> EAGAPCGRISFALRYLYGSDQLVVRILQALDLPAKDSNGFSDPYVKIYLLPDRKKKFQTKVHRKTLNPIFNETFQFSVPLAELAQRKLHFSVYDFDRFSRHDLIGQVVLDNLLELAEQPPDRPLWRDILEGGSEKADLGELNFSLCYLPTAGLLTVTIIKASNLKAMD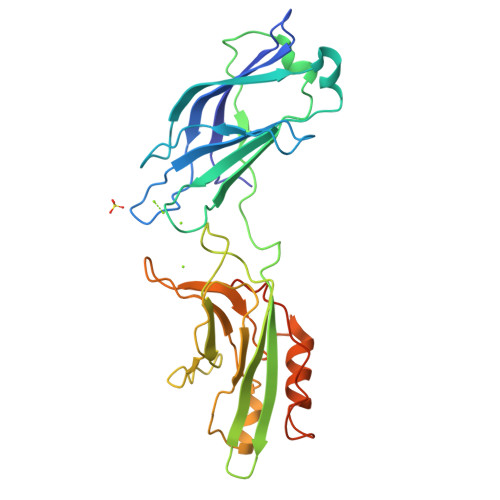LTGFSDPYVKASLISEGRRLKKRKTSIKKNTLNPTYNEALVFDVAPESVENVGLSIAVVDYDCIGHNEVIGVCRVGPEAADPHGREHWAEMLANPRKPVEHWHQLVEEKTLSSFTKGGKGLSEKENSE> GQRIRVRI;> GSVTFEFENLSEEAAEKVKKYVKEVAEKLGVEVKVEEEEGKLKIYVENLKEEDALDIFKYAALAAELDQEYLDMVEAAIKAYHLFKEYDENATIEITIDDEGIEVKVESGDRVVTLKFKNVSKEEVEEAVKEALKQLEAGQ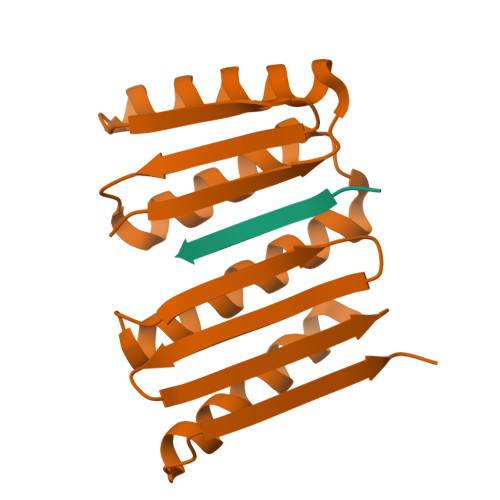KKVEVEVEGGS>GHMEQTHRAIFRFVPRHEDELELEVD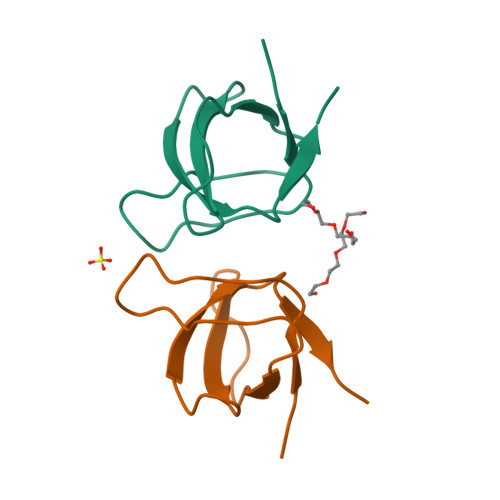DPLLVELQAEDYWYEAYNMRTGARGVFPLYYAIEVTK[4x]(2R)-N-[3-(3,5-dimethylphenyl)-1H-pyrazol-5-yl]-1,4-dioxane-2-carboxamide | C16 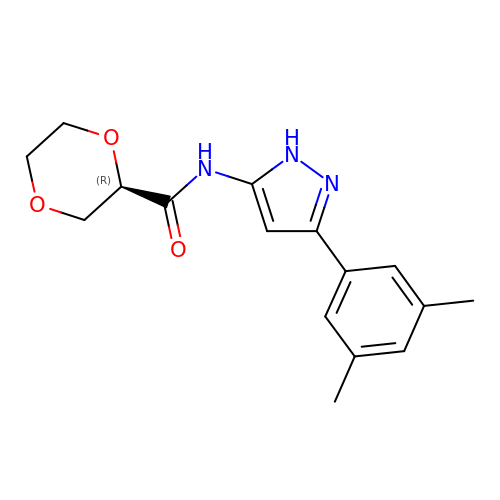H19 N3 O3 | IFBWFTQSSMRHQI-CQSZACIVSA-N> GHM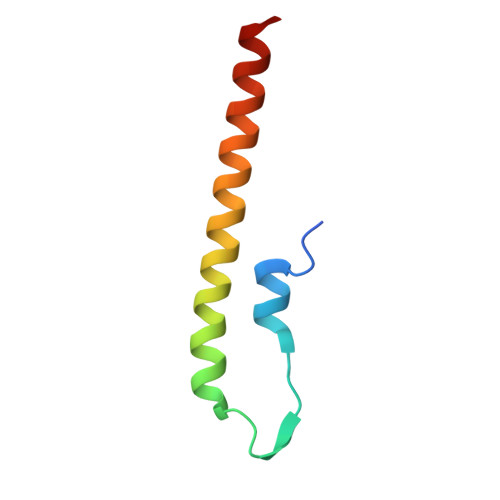KVKLSAKEILEKEFKTGVRGYKQEDVDKFLDMIIKDYETFHQEIEELQQENLQLKKQLEE>MHHHHHHQLHSVGKATQQMMQEPLTKERLISDWNSNVSVAVARTTAIAKSSDASLVQFLAADAAATTKSTANVLKQIEPLITQPAEREILDKIMQVRKTYIASRDKVSQLKADGMAEEAESTLINSYVPAAQGYLKLLGELLNLQ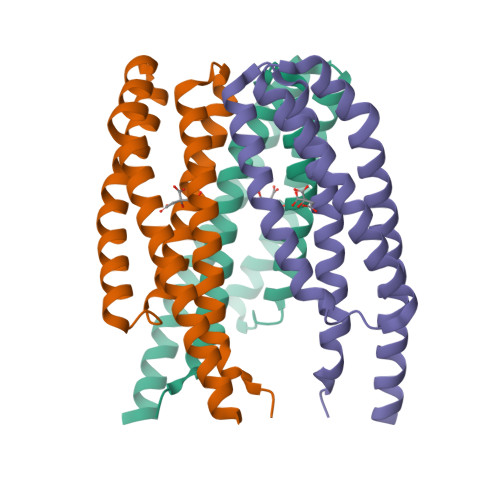RASLDAKAAEVEQIESSSRT[2x]> GHAPDKIVLDHAFGQTILDKKPERVATIAWGNHDVALALGIVPVGFSKANYGVSADKGVLPWTEEKIKELNGKANLFDDLDGLNFEAISNSKPDVILAGYSGITKEDYDTLSKIAPVAAYKSKPWQTLWRDMIKIDSKALGMEKEGDELIKNTEARISKELEKHPEIKGKIKGKKVLFTMINAADTSKFWIYTSKDPRANYLTDLGLVFPESLKEFESEDSFAKEISAEEANKINDADVIITYGDDKTLEALQKDPLLGKINAIKNGAVAVIPDNTPLAASCTPTPLSINYTIEEYLNLLGNA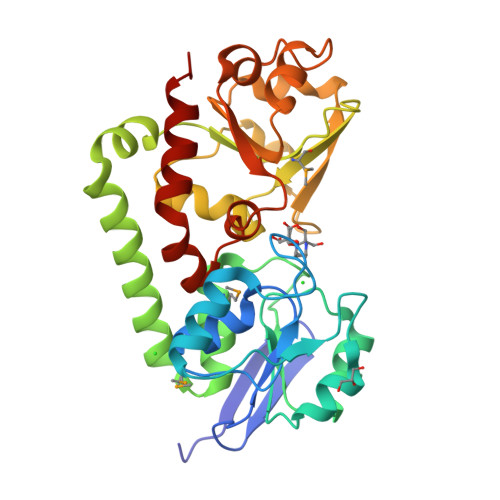CKNAK>[2x]MEQETLEQVHLTEDGGVVKTILRKGEGGEENAPKKGNEVTVHYVGKLESSGKVFDSSRERNVPFKFHLGQGEVIKGWDICVASMTKNEKCSVRLD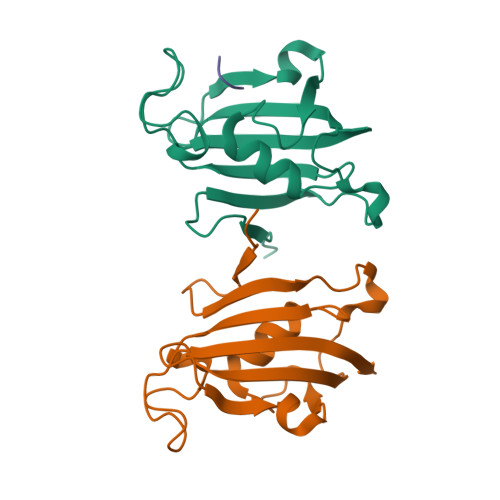SKYGYGEEGCGESIPGNSVLIFEIELISFRE;> ALPF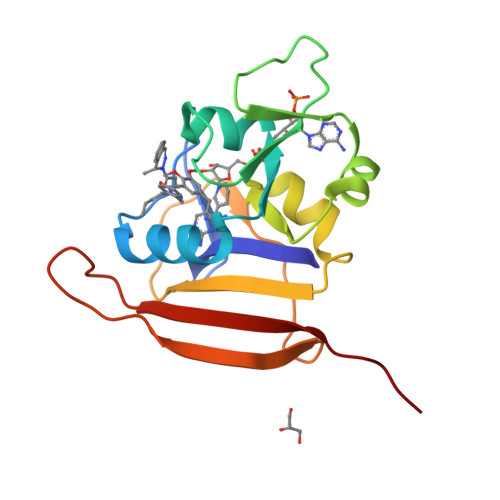> TLSILVAHDLQRVIGFENQLPWHLPNDLKHVKKLSTGHTLVMGRKTFESIGKPLPNRRNVVLTSDTSFNVEGVDVIHSIEDIYQLPGHVFIFGGQTLFEEMIDKVDDMYITVIEGKFRGDTFFPPYTFEDWEVASSVEGKLDEKNTIPHTFLHLIRKAVPR>MFRGSLIAMITPFINGQVDEKALAGLVDWQIKHGAHGLVPVGTTGESPTLTEEEHKRVVALVAEQAQGRVPVIAGAGSNNPVEAVRYAQHAQQAGADAVLCVAGYYNRPSQEGLYQHFKMVHDAIDIPIIVYNIPPRAVVDIKPETMARLAALPRIVGVKDATTDLARISRERMLINKPFSFLSGDDMTAIAYNASGGQGCISVSANIAPALYGQMQTATLQGDFREALRIHDLLAPLHEALFREPSPAGAKYAASLLGLCNEECRLPIVPLSEQTKSDIKNIINELYRL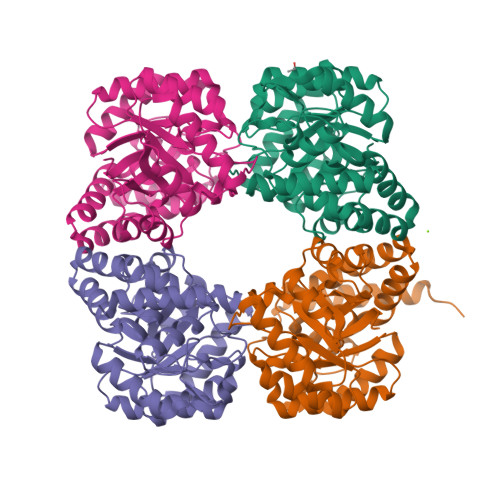EHHHHHH[4x]> AEETSFVFSKFKPLEPNLILQGDALVTVAGVLQLTNVDKNGVPEPSSLGRATYSAPINIWDSATGLVASFATSFRFTIYAPNIATIADGLAFFLAPVASAPDSGGGFLGLF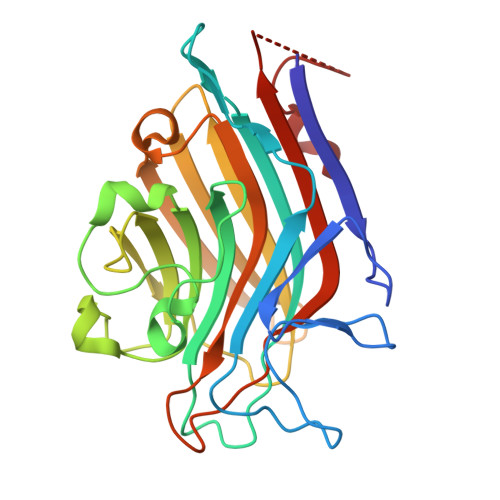DSAVSGSTYQTVAVEFDTYENTVFTDPPYTHIGFDVNSISSIKTVKWSLANGEAAKVLITYNSAVKLLVASLVYPSSKTSFILADIVDLSSVLPEWVRVGFSAATGASGGKIETHDVFSWSFASKLAGXXTKDSSFLDGG>GAMTQGLIEVERKFAPGPDTEERLQELGATLEHRVTFRDTYYDTSELSLMLSDHWLRQREGSGWELKCPGVTGVSGPHNEYVEVTSEAAIVAQLFELLGSGEQKPAGVAAVLGSLKLQEVASFITTRSSWKLALSGAHGQEPQLTIDLDSADFGYAVGEVEAMVHEKAEVPAALEKIITVSSMLGVPAQEEAPAKLMVYLQRFRPLDYQRLLEAA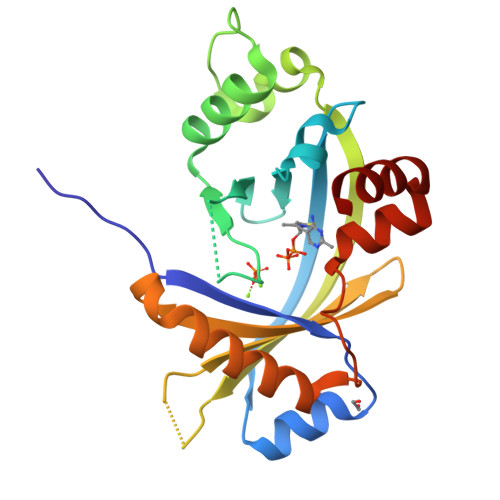SS[2x]>[4x]MIYPIFIFKTVEGFDGYFPDIDGCFFAGNTFADISKNAEEAFAVHIEALMNEGFP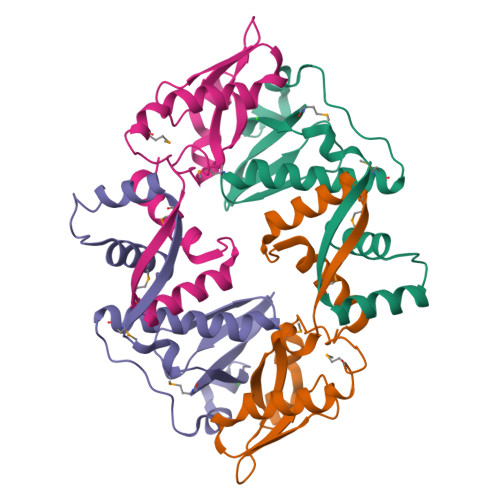LPSPPKDPHRYIDDPRLKEEGGILGFVEIDPAKYESKAVKFNLTMSQNLLTAIDKFIATNRGYKNRSQFLAELAREKIISLEHHHHHH>[3x]MVQTSFEHHHHHHSAGENLYFQGAQISMRLYSNRDRPNHLGPLALERLARVDDVVAQPARQPEDGFAASEDSLLGDVEEYARLFTRFLDGPVAPLGDAIPDDPARRAENLKASAYFLDASMVGICRLDPDDRAGDCDPSHTHALVFAVQFGREPEAGEAGAEWIRGTNAARTDMRCAEIAAILSGYVRWMGFPARGHFSGDAQVDLARLAVRAGLARVVDGVLVAPFLRRGFRLGVVTTGYALAADRPLAPEGDLGETAPEVMLGIDGTRPGWEDAEEEKRPLHMGRYPMETIRRVDEPTTLVVRQEIQRVAKRGDFFKRAEAGDLGEKAKQEKKRFPMKHPLALGMQPLIQNMVPLQGTREKLAPTGKGGDLSDPGRNAEAIKALGYYLGADFVGICRAEPWMYYASDEVEGKPIEAYHDYAVVMLIDQGYETMEGASGDDWISASQSMRAYMRGAEIAGVMAAHCRRMGYSARSHSNAHSEVIHNPAILMAGLGEVSRIGDTLLNPFIGPRSKSIVFTTDLPMSVDRPIDFGLQDFCNQCRKCARECPCNAISFGDKVMFNGYEIWKADVEKCTKYRVTQMKGSACGRCMKMCPWNREDTVEGRRLAELSIKVPEARAAIIAMDDALQNGKRNLIKRWWFDLEVIDGVAGAPRMGTNERDLSPDRGDKIGANQKLAMYPPRLQPPPGTTLDAVLPVDRSGGLAEYAAAETPAAARARLKSSAG

The reductive dehalogenases (RDases) are key enzymes in organohalide respiration, which is performed by a unique subset of bacteria. The RDases are cobalamin-dependent and able to selectively cleave carbon-halogen bonds through reduction. The RDases can be split into two classes: (i) the canonical respiratory dehalogenases, which use a halogenated compound as a final electron acceptor during organohalide respiration and (ii) the catabolic respiratory dehalogenases that occur in the catabolic pathways of non-organohalide respiring bacteria. Structural insight into RDase function is based on two enzymes that have been crystallised, the respiratory perchloroethene (PCE) Sulfurospirillum multivorans reductive dehalogenase (PceA), and the catabolic reductive dehalogenase from Nitratireductor pacificus pht-3B (NpRdhA).

Only one conformation provides a halogen beta axial ligand and thus resembles the 35-DB-4-OH substrate complex (occupancy 30%). One of the two distinct, non-Co-ligating conformations corresponds to that of the previously observed 35-DB-4-OH in crystallo reduction product (occupancy 30%), while the other occupies the entrance of the active site cavity (occupancy 40%). In the latter case, the 3-B-4-OH benzoic acid group forms a salt bridge with K307 (3.1 Å) while the phenolic oxygen interacts with Y426 (2.5 Å). The 3-B-4-OH reductase activity of NpRdhA has previously been shown to be significantly lower (~20%) compared with the 35-DB-4-OH reductase activity. The 3-B-4-OH bound structure reveals this is likely due to multiple conformations, only one of which appears catalytically competent. Indeed, inhibition of NpRdhA reductase activity due to inhibitory substrate binding modes likely accounts for the higher Km and lower kcat seen for this substrate in comparison to 35-DB-4-OH. The lower propensity of 3-B-4-OH to bind in a productive orientation might in part explain the lower activity seen with this substrate in comparison to 35-DB-4-OH.>QLSCTGPPAIPGIPGIPGTPGPDGQPGTPGIKGEKGLPGL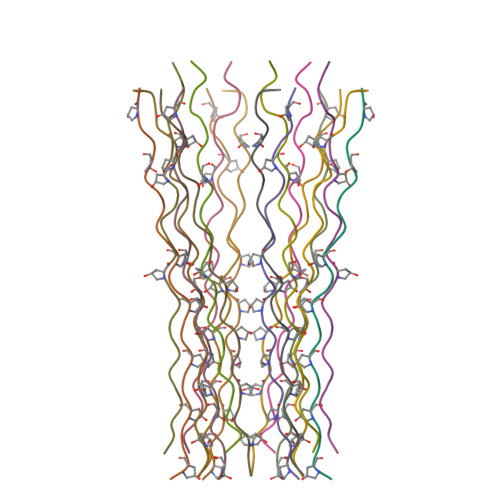AGDH[6x];>[6x]EDLCRAPDGKKGEAGRPGRRGRPGLKGQGEPGAPGIR;>[6x]NTGCYGIPGMPGLPGAPGKDGYDGLPGPKGEPGIP>MGHHHHHMVLADLGRKITSALRSLSNATIINEEVLNAMLKEVCTALLEADVNIKLVKQLRENVKSAIDLEEMASGLNKRKMIQHAVFKE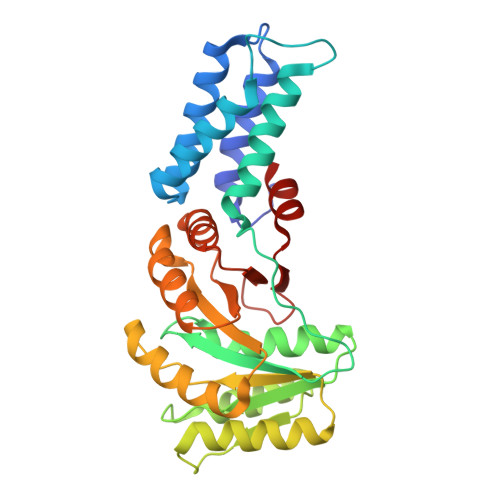LVKLVDPGVKAWTPTKGKQNVIMFVGLQGSGKATTCSKLAYYYQRKGWKTCLICADTFRAGAFDQLKQNATKARIPFYGSYTEMDPVIIASEGVEKFKNENFEIIIVDTSGRHKQEDSLFEEMLQVANAIQPDNIVYVMDASIGQACEAQAKAFKDKVDVASVIVTKLDGHAKGGGALSAVAATKSPIIFIGTGEHIDDFEPFKTQPFISKLLG[2x]>[2x]GGADQKGPVFLKEPTNRIDFSNSTGAEIECKASGNPMPEIIWIRSDGTAVGDVPGLRQISSDGKLVFPPFRAEDYRQEVHAQVYACLARNQFGSIISRDVHVRAVVSQFYITEAENEYVIKGNAAVVKCKIPSFVADFVQVE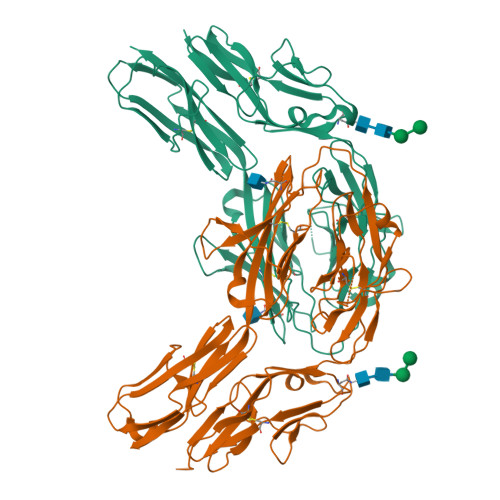AWVDEEGMELWRNNATDAYDGKYLVLPSGELHIREVGPEDGYKSYQCRTKHRLTGETRLSATKGRLVITEPVGSVSPQLSGNGNQEHITLTRVPKMGSVTLMCPAQAYPVPFFRWYKFIEGTTRKQAVVLNDRVKQVSGTLIIKDAVVEDSGKYLCVVNNSVGGESVETVLTVTAPLSAKIDPPTQTVDFGRPAVFTCQYTGNPIKTVSWMKDGKAIGHSEPVLRIESVKKEDKGMYQCFVRNDQESAEASAELKLGG>MSPIPNRVSSGSLADAVFKSACEERILLAYADYNPDMTKVVNLFSKYNETVNTVRVSNDAVKDILEIVGWPSMPLIFVKGNCCGGFKELYQLEESGFLNEWLKEHEYDLAIVGGGSGGLAAAKEAVRLGKKVVCLDFVKPSAMGTTWGLGGTCVNVGCIPKKLMHQAALLGEYIEDAKKFGWEIPEGAIKLNWHQLKNAVQNHIASLNWGYRV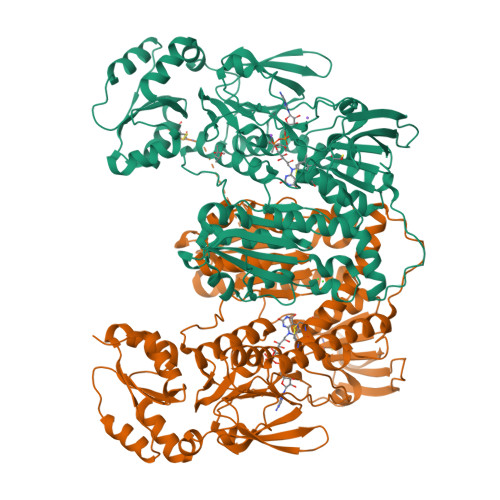QLKEKSVTYMNSYATFTGSHELSVKNKKGKVEKVTADRFLIAVGLRPRFPDVPGALECCISSDDLFSLPYNPGKTLCVGASYVSLECAGFLKGIGNDVTVMVRSVLLRGFDQDMAERIKKHMTERGVKFVQCVPIKYERLKKPTDSEPGMIRVHTMQEDEDGTKEVTEDFNTVLMAIGRDAMTDDLGLDVVGVNRAKSGKIIGRREQSVSCPYVYAIGDVLYGSPELTPVAIQAGKVLMRRLFTGSSELTEYDKIPTTVFTPLEYGSCGLSEYSAIQKYGKENINVYHNVFIPLEYAVTERKEKTHCYCKLICLKNEQDLILGFHILTPNAGEITQGFAIALKFDAKKADFDRLIGIHPTVAENFTTLTLVKEDGQTLKATGCUG[3x]>GASGSGSGMLEVCIIGFGFSAIPLVRELARTQTEFQIISAESGSVWDRLSESGRLDFSLVSSFQTSFYSFDLVRDYEKDYYPTAKQFYEMHERWRSVYEEKIIRDFVTKIENFKDYSLISTRSGKTYEAKHVVLATGFDRLMNTFLSNFDNHVSNKTFVFDTMGDSANLLIAKLIPNNNKIILRTNGFTALDQEVQVLGKPFTLDQLESPNFRYVSSELYDRLMMSPVYPRTVNPAVSYNQFPLIRRDFSWVDSKSSPPNGLIAIKYWPIDQYYYHFNDDLENYISKGYLLNDIAMWLHTGKVILVPSDTPINFDKKTITYAGIERSFHQYVKGDAEQPRLPTILINGETPFEYLYRDTFMGVIPQRLNNIYFLGYTRPFTGGLANITEMQSLFIHKLITQPQFHQKIHQNLSKRITAYNQHYYGAAKPRKHDHTVPFGFYTEDIARLIGIHYQPNECRSVRDLLFYYAFPNNAFKYRLKGEYAVDGVDELIQKVNDKHDHYAQVFVQALSIRNMNSDEAAEWDHSARRFSFNDMRHKEGYRAFLDTYLKAYRQVENISVDDTVVDEEWNFMVKEACQVRDKVAPNIEEKTHYSKDEDVNKGIRLILSILDSDISSLPDSNGSRGSGNLKEGDRLCKFEAQSIEFIRRLLQPKNYELLFIRES[2x]

The flavin-dependent halogenase (FDH) AetF successively brominates tryptophan at C5 and C7 to generate 5,7-dibromotryptophan. In contrast to the well studied two-component tryptophan halogenases, AetF is a single-component flavoprotein monooxygenase. A large domain tightly binds the cofactor flavin adenine dinucleotide (FAD), while the small domain responsible for binding the nicotinamide adenine dinucleotide (NADP) is unoccupied. About half of the protein forms additional structural elements containing the tryptophan binding site.

Structure determination was straightforward for non-substrate-bound (empty AetF) and 5-Br-Trp-bound AetF (AetF–5-Br-Trp). These crystals were isomorphous to each other and scaled in space groups P41 or P43 without signs of twinning or translational noncrystallographic symmetry (tNCS). The structure of AetF co-crystallized with 5-Br-Trp was phased by the difference Fourier method. In the case of 5-Br-Trp, the position of the Br atom could be unambiguously determined based on the anomalous difference density. The indole moiety of 5-Br-Trp lies in the same plane as that of Trp but is flipped around an axis formed by C3 and C6, the positions of which are almost unchanged, while N1, C2, C5 and C7 are rotated by ∼180° around this axis. The indole moiety of 5-Br-Trp is surrounded by the same hydrophobic (Leu183, Leu196, Met216, Pro219, Phe373 and Phe524) and polar (Glu200 and Thr373) residues as that of Trp, but its NH group now forms a hydrogen bond to the carbonyl of Leu196 instead of Met216. The side chain of Gln500, which binds both the amino and the carboxy group of Trp, rearranges and its amide group flips so that it can again form hydrogen bonds to both the amino and carboxy groups of 5-Br-Trp. The flipped binding pose of 5-Br-Trp leads to an almost congruent position of the C atoms that will be halogenated in the two substrates. C5 of Trp and C7 of 5-Br-Trp are less than 0.5 Å apart when overlaying the two structures This suggests that C5 of Trp and C7 of 5-Br-Trp will be positioned productively relative to the catalytic residues.>[4x]MFPAAPSPRTPGTGSRRGPLAGLGPGSTPRTASRKGLPLGSAVSSPVLFSPVGRRSSLSSRGTPTRMFPHHSITESVNYDVKTFGSSLPVKVMEALTLAEVDDQLTINIDEGGWACLVCKEKLIIWKIALSPITKLSVCKELQLPPSDFHWSADLVALSYSSPSGEAHSTQAVAVMVATREGSIRYWPSLAGEDTYTEAFVDSGGDKTYSFLTAVQGGSFILSSSGSQLIRLIPESSGKIHQHILPQGQGMLSGIGRKVSSLFGILSPSSDLTLSSVLWDRERSSFYSLTSSNISKWELDDSSEKHAYSWDINRALKENITDAIWGSESNYEAIKEGVNIRYLDLKQNCDGLVILAAAWHSADNPCLIYYSLITIEDNGCQMSDAVTVEVTQYNPPFQSEDLILCQLTVPNFSNQTAYLYNESAVYVCSTGTGKFSLPQEKIVFNAQGDSVLGAGACGGVPIIFSRNSGLVSITSRENVSILAEDLEGSLASSVAGPNSESMIFETTTKNETIAQEDKIKLLKAAFLQYCRKDLGHAQMVVDELFSSHSDLDSDSELDRAVTQISVDLMDDYPASDPRWAESVPEEAPGFSNTSLIILHQLEDKMKAHSFLMDFIHQVGLFGRLGSFPVRGTPMATRLLLCEHAEKLSAAIVLKNHHSRLSDLVNTAILIALNKREYEIPSNLTPADVFFREVSQVDTICECLLEHEEQVLRDAPMDSIEWAEVVINVNNILKDMLQAASHYRQNRNSLYRREESLEKEPEYVPWTATSGPGGIRTVIIRQHEIVLKVAYPQADSNLRNIVTEQLVALIDCFLDGYVSQLKSVDKSSNRERYDNLEMEYLQKRSDLLSPLLSLGQYLWAASLAEKYCDFDILVQMCEQTDNQSRLQRYMTQFADQNFSDFLFRWYLEKGKRGKLLSQPISQHGQLANFLQAHEHLSWLHEINSQELEKAHATLLGLANMETRYFAKKKTLLGLSKLAALASDFSEDMLQEKIEEMAEQERFLLHQETLPEQLLAEKQLNLSAMPVLTAPQLIGLYICEENRRANEYDFKKALDLLEYIDEEEDININDLKLEILCKALQRDNWSSSDGKDDPIEVSKDSIFVKILQKLLKDGIQLSEYLPEVKDLLQADQLGSLKSNPYFEFVLKANYEYYVQGQI;>[4x]MDRSGFGEISSPVIREAEVTRTARKQSAQKRVLLQASQDENFGNTTPRNQVIPRTPSSFRQPFTPTSRSLLRQPDISCILGTGGKSPRLTQSSGFFGNLSMVTNLDDSNWAAAFSSQRSGLFTNTEPHSITEDVTISAVMLREDDPGEAASMSMFSDFLQSFLKHSSSTVFDLVEEYENICGSQVNILSKIVSRATPGLQKFSKTASMLWLLQQEMVTWRLLASLYRDRIQSALEEESVFAVTAVNASEKTVVEALFQRDSLVRQSQLVVDWLESIAKDEIGEFSDNIEFYAKSVYWENTLHTLKQRQLTSYVGSVRPLVTELDPDAPIRQKMPLDDLDREDEVRLLKYLFTLIRAGMTEEAQRLCKRCGQAWRAATLEGWKLYHDPNVNGGTELEPVEGNPYRRIWKISCWRMAEDELFNRYERAIYAALSGNLKQLLPVCDTWEDTVWAYFRVMVDSLVEQEIQTSVATLDETEELPREYLGANWTLEKVFEELQATDKKRVLEENQEHYHIVQKFLILGDIDGLMDEFSKWLSKSRNNLPGHLLRFMTHLILFFRTLGLQTKEEVSIEVLKTYIQLLIREKHTNLIAFYTCHLPQDLAVAQYALFLESVTEFEQRHHCLELAKEADLDVATITKTVVENIRKKDNGEFSHHDLAPALDTGTTEEDRLKIDVIDWLVFDPAQRAEALKQGNAIMRKFLASKKHEAAKEVFVKIPQDSIAEIYNQCEEQGMESPLPAEDDNAIREHLCIRAYLEAHETFNEWFKHMNSVPQKPALIPQPTFTEKVAHEHKEKKYEMDFGIWKGHLDALTADVKEKMYNVLLFVDGGWMVDVREDAKEDHERTHQMVLLRKLCLPMLCFLLHTILHSTGQYQECLQLADMVSSERHKLYLVFSKEELRKLLQKLRESSLMLLDQGLDPLGYEIQL;>SKYGLQDSDEEEEEHPSKTSTKKLKTAPLPPASQTTPLQMALNGKPAPPPQSQSPEVEQLGRVVELDSDMVDITQEPVLDTMLEESMPEDQEPVSASTHIASSLGINPHVLQIMKASLLTDEEDVDMALDQRFSRLPSKADTSQEICSPRLPISASHSSKTRSLVGGLLQSKFTSGAFLSPSVSVQECRTPRAASLMNIPSTSSWSVPPPLTSVFTMPSPAPEVPLKTVGTRRQLGLVPREKSVTYGKGKLLMDMALFMGRSFRVGWGPNWTLANSGEQLNGSHELENHQIADSMEFGFLPNPVAVKPLTESPFKVHLEKLSLRQRKPDEDMKLYQTPLELKLKHSTVHVDELCPLIVPNLGVAVIHDYADWVKEASGDLPEAQIVKHWSLTWTLCEALWGHLKELDSQLNEPREYIQILERRRAFSRWLSCTATPQIEEEVSLTQKNSPVEAVFSYLTGKRISEACSLAQQSGDHRLALLLSQFVGSQSVRELLTMQLVDWHQLQADSFIQDERLRIFALLAGKPVWQLSEKKQINVCSQLDWKRSLAIHLWYLLPPTASISRALSMYEEAFQNTSDSDRYACSPLPSYLEGSGCVIAEEQNSQTPLRDVCFHLLKLYSDRHYDLNQLLEPRSITADPLDYRLSWHLWEVLRALNYTHLSAQCEGVLQASYAGQLESEGLWEWAIFVLLHIDNSGIREKAVRELLTRHCQLLETPESWAKETFLTQKLRVPAKWIHEAKAVRAHMESDKHLEALCLFKAEHWNRCHKLIIRHLASDAIINENYDYLKGFLEDLAPPERSSLIQDWETSGLVYLDYIRVIEMLRHIQQVDCSGNDLEQLHIKVTSLCSRIEQIQCYSAKDRLAQSDMAKRVANLLRVVLSLHHPPDRTSDSTPDPQRVPLRLLAPHIGRLPMPEDYAMDELRSLTQSYLRELAVGSL[4x];>[4x]MVSVINTVDTSHEDMIHDAQMDYYGTRLATCSSDRSVKIFDVRNGGQILIADLRGHEGPVWQVAWAHPMYGNILASCSYDRKVIIWREENGTWEKSHEHAGHDSSVNSVCWAPHDYGLILACGSSDGAISLLTYTGEGQWEVKKINNAHTIGCNAVSWAPAVVPGSLIDHPSGQKPNYIKRFASGGCDNLIKLWKEEEDGQWKEEQKLEAHSDWVRDVAWAPSIGLPTSTIASCSQDGRVFIWTCDDASSNTWSPKLLHKFNDVVWHVSWSITANILAVSGGDNKVTLWKESVDGQWVCISDVNKGQGSVSASVTEGQQNEQ;>MFVARSIAADH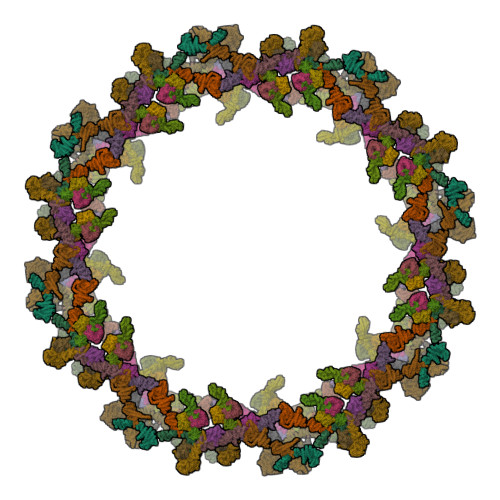KDLIHDVSFDFHGRRMATCSSDQSVKVWDKSESGDWHCTASWKTHSGSVWRVTWAHPEFGQVLASCSFDRTAAVWEEIVGESNDKLRGQSHWVKRTTLVDSRTSVTDVKFAPKHMGLMLATCSADGIVRIYEAPDVMNLSQWSLQHEISCKLSCSCISWNPSSSRAHSPMIAVGSDDSSPNAMAKVQIFEYNENTRKYAKAETLMTVTDPVHDIAFAPNLGRSFHILAIATKDVRIFTLKPVRKELTSSGGPTKFEIHIVAQFDNHNSQVWRVSWNITGTVLASSGDDGCVRLWKANYMDNWKCTGILKGNGSPVNGSSQQGTSNPSLGSTIPSLQNSLNGSSAGRKHS[4x];>[4x]MEELDGEPTVTLIPGVNSKKNQMYFDWGPGEMLVCETSFNKKEKSEMVPSCPFIYIIRKDVDVYSQILRKLFNESHGIFLGLQRIDEELTGKSRKSQLVRVSKNYRSVIRACMEEMHQVAIAAKDPANGRQFSSQVSILSAMELIWNLCEILFIEVAPAGPLLLHLLDWVRLHVCEVDSLSADVLGSENPSKHDSFWNLVTILVLQGRLDEARQMLSKEADASPASAGICRIMGDLMRTMPILSPGNTQTLTELELKWQHWHEECERYLQDSTFATSPHLESLLKIMLGDEAALLEQKELLSNWYHFLVTRLLYSNPTVKPIDLHYYAQSSLDLFLGGESSPEPLDNILLAAFEFDIHQVIKECSIALSNWWFVAHLTDLLDHCKLLQSHNLYFGSNMREFLLLEYASGLFAHPSLWQLGVDYFDYCPELGRVSLELHIERIPLNTEQKALKVLRICEQRQMTEQVRSICKILAMKAVRNNRLGSALSWSIRAKDAAFATLVSDRFLRDYCERGCFSDLDLIDNLGPAMMLSDRLTFLGKYREFHRMYGEKRFADAASLLLSLMTSRIAPRSFWMTLLTDALPLLEQKQVIFSAEQTYELMRCLEDLTSRRPVHGESDTEQLQDDDIETTKVEMLRLSLARNLARAIIREGSLEGS;>[4x]MEEIYAKFVSQKISKTRWRPLPPGSLQTAETFATGSWDNEENYISLWSIGDFGNLDSDGGFEGDHQLLCDIRHHGDVMDLQFFDQERIVAASSTGCVTVFLHHPNNQTLSVNQQWTTAHYHTGPGSPSYSSAPCTGVVCNNPEIVTVGEDGRINLFRADHKEAVRTIDNADSSTLHAVTFLRTPEILTVNSIGQLKIWDFRQQGNEPSQILSLTGDRVPLHCVDRHPNQQHVVATGGQDGMLSIWDVRQGTMPVSLLKAHEAEMWEVHFHPSNPEHLFTCSEDGSLWHWDASTDVPEKSSLFHQGGRSSTFLSHSISNQANVHQSVISSWLSTDPAKDRIEITSLLPSRSLSVNTLDVLGPCLVCGTDAEAIYVTRHLFS;>MLHLSAAPPAPPPEVTATARPCLCSVGRRGDGGKMAAAGALERSFVELSGAERERPRHFREFTVCSIGTANAVAGAVKYSESAGGFYYVESGKLFSVTRNRFIHWKTSGDTLELMEESLDINLLNNAIRLKFQNCSVLPGGVYVSETQNRVIILMLTNQTVHRLLLPHPSRMYRSELVVDSQMQSIFTDIGKVDFTDPCNYQLIPAVPGISPNSTASTAWLSSDGEALFALPCASGGIFVLKLPPYDIPGMVSVVELKQSSVMQRLLTGWMPTAIRGDQSPSDRPLSLAVHCVEHDAFIFALCQDHKLRMWSYKEQMCLMVADMLEYVPVKKDLRLTAGTGHKLRLAYSPTMGLYLGIYMHAPKRGQFCIFQLVSTESNRYSLDHISSLFTSQETLIDFALTSTDIWALWHDAENQTVVKYINFEHNVAGQWNPVFMQPLPEEEIVIRDDQDPREMYLQSLFTPGQFTNEALCKALQIFCRGTERNLDLSWSELKKEVTLAVENELQGSVTEYEFSQEEFRNLQQEFWCKFYACCLQYQEALSHPLALHLNPHTNMVCLLKKGYLSFLIPSSLVDHLYLLPYENLLTEDETTISDDVDIARDVICLIKCLRLIEESVTVDMSVIMEMSCYNLQSPEKAAEQILEDMITIDVENVMEDICSKLQEIRNPIHAIGLLIREMDYETEVEMEKGFNPAQPLNIRMNLTQLYGSNTAGYIVCRGVHKIASTRFLICRDLLILQQLLMRLGDAVIWGTGQLFQAQQDLLHRTAPLLLSYYLIKWGSECLATDVPLDTLESNLQHLSVLELTDSGALMANRFVSSPQTIVELFFQEVARKHIISHLFSQPKAPLSQTGLNWPEMITAITSYLLQLLWPSNPGCLFLECLMGNCQYVQLQDYIQLLHPWCQVNVGSCRFMLGRCYLVTGEGQKALECFCQAASEVGKEEFLDRLIRSEDGEIVSTPRLQYYDKVLRLLDVIGLPELVIQLATSAITEAGDDWKSQATLRTCIFKHHLDLGHNSQAYEALTQIPDSSRQLDCLRQLVVVLCERSQLQDLVEFPYVNLHNEVVGIIESRARAVDLMTHNYYELLYAFHIYRHNYRKAGTVMFEYGMRLGREVRTLRGLEKQGNCYLAALNCLRLIRPEYAWIVQPVSGAVYDRPGASPKRNHDGECTAAPTNRQIEILELEDLEKECSLARIRLTLAQHDPSAVAVAGSSSAEEMVTLLVQAGLFDTAISLCQTFKLPLTPVFEGLAFKCIKLQFGGEAAQAEAWAWLAANQLSSVITTKESSATDEAWRLLSTYLERYKVQNNLYHHCVINKLLSHGVPLPNWLINSYKKVDAAELLRLYLNYDLLEEAVDLVSEYVDAVLGKGHQYFGIEFPLSATAPMVWLPYSSIDQLLQALGENSANSHNIALSQKILDKLEDYQQKVDKATRDLLYRRTL[4x];>MKQDASRNAAYTVDCEDYVHVVEFNPFENGDSGNLIAYGGNNYVVIGTCTFQEEEADVEGIQYKTLRTFHHGVRVDGIAWSPETRLDSLPPVIKFCTSAADMKIRLFTSDLQDKNEYKVLEGHTDFINGLVFDPKEGQEIASVSDDHTCRIWNLEGVQTAHFVLHSPGMSVCWHPEETFKLMVAEKNGTIRFYDLLAQQAILSLESEQVPLMSAHWCLKNTFKVGAVAGNDWLIWDITRSSYPQNKRPVHMDRACLFRWSTISENLFATTGYPGKMASQFQIHHLGHPQPILMGSVAVGSGLSWHRTLPLCVIGGDHKLLFWVTEV[4x]> MKKRLTESQFQEAIQGLEVGQQTIEIARGVLVDGKPQATFATSLGLTRGAVSQAVHRVWAAFEDKNLPEGYARVTAVLPEHQ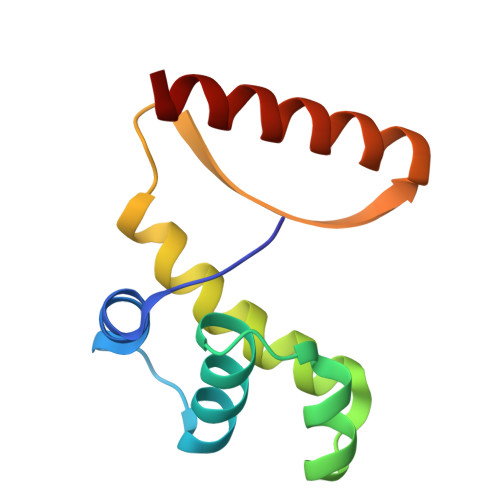AYIVRKWEADAKKKQET> GPRQWALEDFEIGRPLGKGKFGNVYLAREKQSKFILALKVLFKAQLE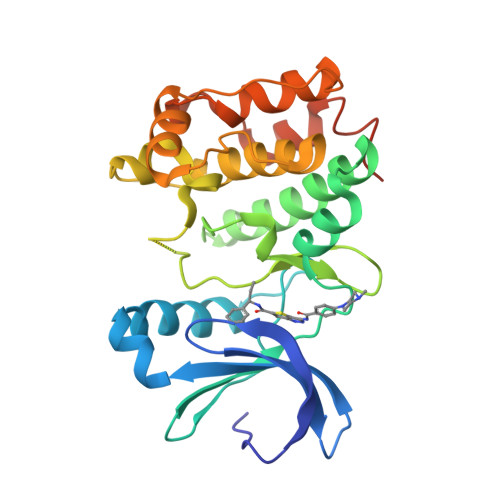KAGVEHQLRREVEIQSHLRHPNILRLYGYFHDATRVYLILEYAPLGTVYRELQKLSKFDEQRTATYITELANALSYCHSKRVIHRDIKPENLLLGSAGELKIADFGWSVHAPSSRRTELCGTLDYLPPEMIEGRMHDEKVDLWSLGVLCYEFLVGKPPFEANTYQETYKRISRVEFTFPDFVTEGARDLISRLLKHNPSQRPMLREVLEHPWITANSSKPSNCQNKESASKQS> MIFSVDKVRADFPVLSREVNGLPLAYLDSAASAQKPSQVIDAEAEFYRHGYAAVHRGIHTLSAQATEKMENVRKRASLFINARSAEELVFVRGTTEGIALVANSWGNSNVRAGDNIIISQMEHHANIVPWQMLCARVGAELRVIPLNPDGTLQLETLPTLFDEKTRLLAITHVSNVLGTENPLAEMITLAHQHGAKVLVDGAQAVMHHPVDVQALDCDFYVFSGHKLYGPTGIGILYVKEALLQEMPPWEGGGSMIATVSLSEGTTWTKAPWRFEAGTPNTGGIIGLGAALEYVSALGLNNIAEYEQNLMHYALSQLESVPDLTLYGPQNRLGVIAFNLGKHHAYDVGSFLDNYGIAVRTGHHCAMPLMAYYNVPAMCRASLAMYNTHEEVDRLVTGLQRIHRLLG

SufS is a pyridoxal-5′-phosphate–dependent enzyme that uses cysteine to generate alanine and an active-site persulfide (C364-S-S-). The SufS persulfide is protected from external oxidants/reductants and requires the transpersulfurase, SufE, to accept the persulfide to complete the SufS catalytic cycle. The β-latch contains four key components: the α6 helix, a glycine-rich loop, a β-hairpin, and a cis-proline. R92 and E96 (E. coli numbering) form cross-dimer electrostatic interactions with the α6 helix of the adjacent monomer, and N99 forms hydrogen bonds to the backbone amide and carbonyl of G251 in the glycine-rich loop.

We generated variants of SufS with either alanine or aspartate at position N99 and solved the crystal structures of the resulting proteins. Alteration of N99 results in significant, but localized, perturbations in components of the β-latch structural element. The structure of N99A SufS has continuous electron density for the β-latch; however, the glycine-rich loop and β-hairpin are shifted, exposing the SufS active site to solvent. In contrast to N99D, the N99A SufS structure does not show disruption of the cross-dimer interactions between R92 and E96. In the N99A SufS structure density for the glycine-rich loop and the β-hairpin is seen, suggesting they are less dynamic and are still capable of physically blocking the active site from solvent. However, the glycine-rich loop is in an altered conformation compared with the WT SufS structure. This altered conformation shifts the position of the S254 amide away from the active site by over 8 Å. The backbone amide of S254 has been shown to interact with the terminal sulfur of the C364 persulfide in the outward-facing position. Loss of this interaction could affect the stability of the persulfide intermediate to nucleophilic attack.> AERPTLPIPDLLTTDARNRIQLTIGAGQSTFGGKTATTWGYNGNLLGPAVKLQRGKAVTVDIYNQLTEETTLHWHGLEVPGEVDGGPQGIIPPGGKRSVTLNVDQPAATCWFHPHQHGKTGRQVAMGLAGLVVIEDDEILKLMLPKQWGIDDVPVIVQDKKFSADGQIDYQLDVMTAAVGWFGDTLLTNGAIYPQHAAPRGWLRLRLLNGCNARSLNFATSDNRPLYVIASDGGLLPEPVKVSELPVLMGERFEVLVEVNDNKPFDLVTLPVSQMGMAIAPFDKPHPVMRIQPIAISASGALPDTLSSLPALPSLEGLTVRKL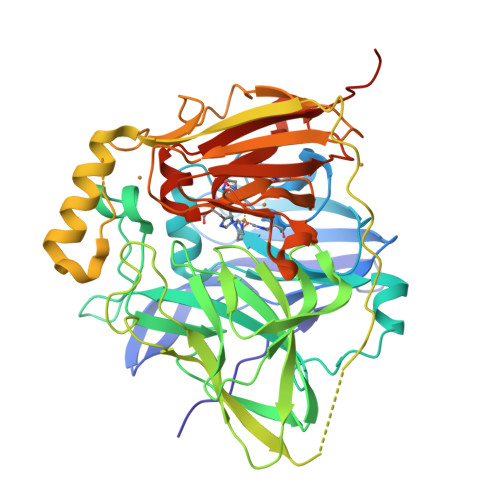QLSMDPSLDSSGSQSLSEKYGDQAMAGMDHSQMMGHMGHGNMNHMNHGGKFDFHHANKINGQAFDMNKPMFAAAKGQYERWVISGVGDMMLHPFHIHGTQFRILSENGKPPAAHRAGWKDTVKVEGNVSEVLVKFNHDAPKEHAYMAHCHLLEHEDTGMMLGFTVLQGDHGLQGDHGLSAWSHPQFEK> MVSTQNEPHRFPPDFQWGVATSSYQIEGAVEADGRSPSIWDTFCARPGAIADGSTGAIANDHYHRYREDIAIMKQLGVNAYRFSIAWPRILPDGRGRVNQAGVDFYERLVDSLLEQGIEPYATLYHWDMPQVQHDRTPWYDRGVVDAFVEYTDVITRRLSDRVKYWMTLNEPWVISFLGYGAGEHAPGLRDKELYLRAAHHVLLAHGKAMPVI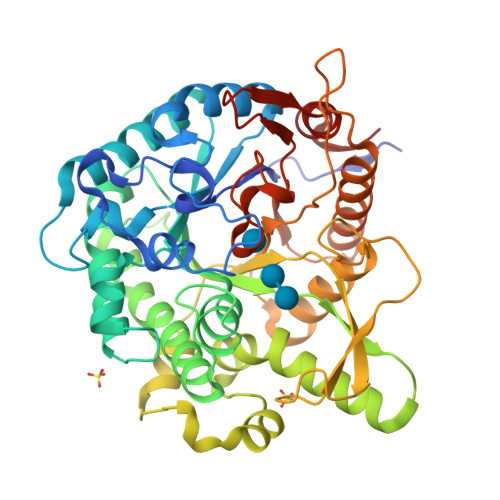RANGNAQTKAGIVLNLNWVNAASDSPEDQAAARRYDQFFNRWFAEPLYNGRYPEELLEWYGRDLVPVQPGDFDIITTPTDFLAVNYYARTTVKAGSTDPMLQVDFVRPPGEYTAMDWEVYPQGLYNILNWLHTDYAPPALYVTENGAAYDDQVSAAGEVDDPQRLAYLEGHFEAAYRAIQAGIPLKGYFVWSLMDNFEWGRGFEKRFGIVFVDYATQQRIIKRSGKWFSQVTRANGLPAPQTTLP Members of the Vaccinia-related kinase (VRK) family of serine/threonine protein kinases are present in the genomes of all metazoans and those of poxviruses, including the family-founding member vaccinia virus B1R1–6. Here we present the first crystal structures of the kinase domain of VRK1 and the first crystal structures for ligand-bound VRK1 and VRK2. Ligand-bound VRK kinase domains adopt the canonical protein kinase fold, except for the presence of the additional α-helix between αC and β4 (αC4) exclusively found on VRK proteins. The ligand-bound structures obtained here for active VRKs are in a closed, active conformation and display the same overall organization previously observed for the apo-structures, including the position of the VRK-exclusive αC4 and the structural organization of conserved residues that make up the kinase hydrophobic spine36.

To understand the ligand binding site of active VRK proteins, we crystallized them in the presence of BI-D1870, the top DSF hit from the commercial library identified here. The most complete VRK13-364/ASC24 model contains residues 21–46 and 48–341 (chain A); and the one for the VRK13-364/BI-D1870 complex contains residues 20–43, 49–341 (chain A). Moreover, the co-structure of VRK13-364 bound to BI-D1870 revealed this compound cannot stabilize a P-loop folded conformation in this protein. Finally, BI-D1870 is seen in two different poses, supported by distinct hinge-binding modes. Both poses only loosely complement the volume of the ATP-binding pocket and neither pose induced the folded P-loop conformation, most likely due to steric effects with P-loop residue Phe48. Structural comparisons of the solution NMR structure, where residues (346–354) within the C-terminal regulatory tail occupy the ATP-binding pocket, and the ligand-bound VRK1 structures obtained here reveal that changes in the ATP-binding site are mostly limited to the protein DYG motif and to the P-loop. Overall, binding of small molecule inhibitors to VRK1 repositioned the catalytic lysine to facilitate the formation of an ion pair between this residue and the conserved glutamate residue from αC, one of the hallmarks of the kinase active conformation. Our data show that BI-D1870 also targets the active VRKs and that this compound could serve as an advanced starting point for a specific inhibitor of these proteins.

>[4x]SMRVKAAQAGRQSSAKRHLAEQFAVGEIITDMAAAAWKVGLPIGQGGFGCIYLADMNSSESVGSDAPCVVKVEPSDNGPLFTELKFYQRAAKPEQIQKWIRTRKLKYLGVPKYWGSGLHDKNGKSYRFMIMDRFGSDLQKIYEANAKRFSRKTVLQLSLRILDILEYIHEHEYVHGDIKASNLLLNYKNPDQVYLVDYGLAYRYCPEGVHKAYAADPKRCHDGTIEFTSIDAHNGVAPSRRGDLEILGYCMIQWLTGHLPWEDNLKDPKYVRDSKIRYRENIASLMDKCFPAANAPGEIAKYMETVKLLDYTEKPLYENLRDILLQGLKAIGSKDDGKLDLSVVENGGLKAKTITKKRAAEIEE> MMANRMILNETAWFGRGAVGALTDEVKRRGYQKALIVTDKTLVQCGVVAKVTDKMDAAGLAWAIYDGVVPNPTI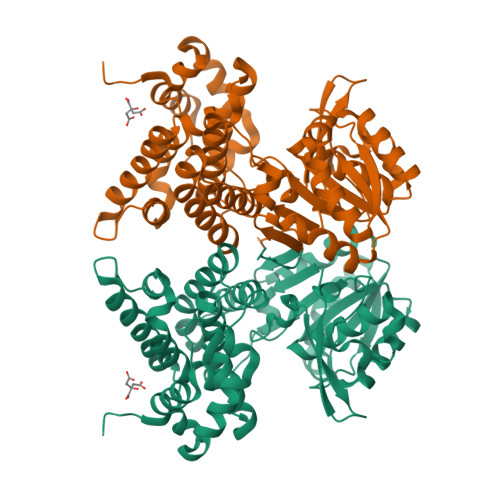TVVKEGLGVFQNSGADYLIAIGGGSPQDTCKAIGIISNNPEFADVRSLEGLSPTNKPSVPILAIPTTAGTAAEVTINYVITDEEKRRKFVCVDPHDIPQVAFIDADMMDGMPPALKAATGVDALTHAIEGYITRGAWALTDALHIKAIEIIAGALRGSVAGDKDAGEEMALGQYVAGMGFSNVGVGLVHGMAHPLGAFYNTPHGVANAILLPHVMRYNADFTGEKYRDIARVMGVKVEGMGLEEARNAAVEAVFALNRDVGIPPHLRDVGVRKEDIPALAQAALDDVCTGGNPREATLEDIVELYHTAWTSHHHHH> MILSSLLPLSLVTLTSAALTYRGADISSLLIEEDSGVAYKNLNGETQAFELILANNGVNSIRQRIWVNPSDGSYNLEYNLELAKRVQDAGMSVYLDLHLSDTWADPGDQATPSGWSTTDIDTLAWQVYNYTLDVCNTFAENNVAVEIVSIGNEIRNGLLHPLGSTDHYDNIARLLHSGAWGVKDSSLSTTPKILFHLDNGWDWDAQKYFYDTVLATGTLLSTDFDLIGVSYYPFYNADATLSSLKTSLTNLKSNYGKNVLVVETDWPVQCSSPEYAFPSDLSSIPFSADGQETFLGRLADTLEDVGGVGIYYWEPGW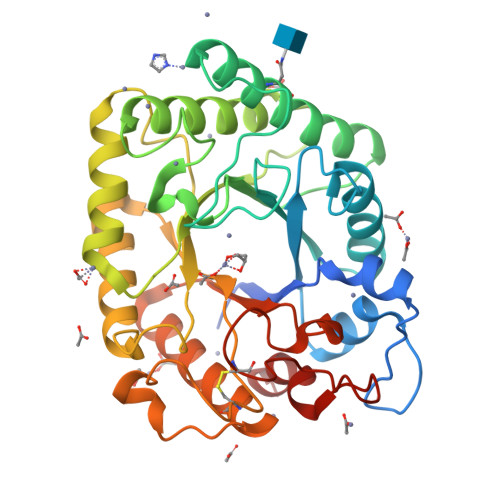VDNAGLGSSCEDNLMVDWRDRTVRESISVFGDLAA> MERPKLGLIVREPYASLIVDGRKVWEIRRRKTRHRGPLGIVSGGRLIGQADLVGVEGPFSVEELLAHQEKHLAEEAFLRAYAKDEPLYAWVL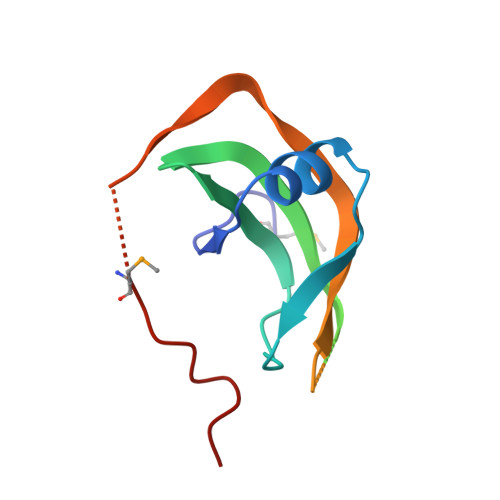ENAFRYEKPLHVPRRPGRVMFVDLSEVRW> GSHMSPREQDRFLPIANVS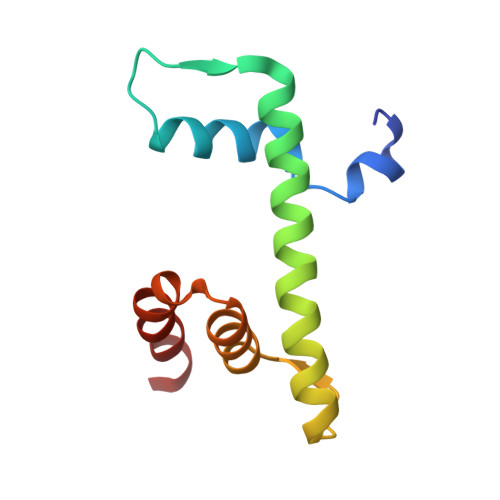RIMKKALPANAKISKDAKETMQECVSEFISFVTGEASDKCQKEKRKTINGDDLLWAMTTLGFEDYVEPLKVYLQRFRE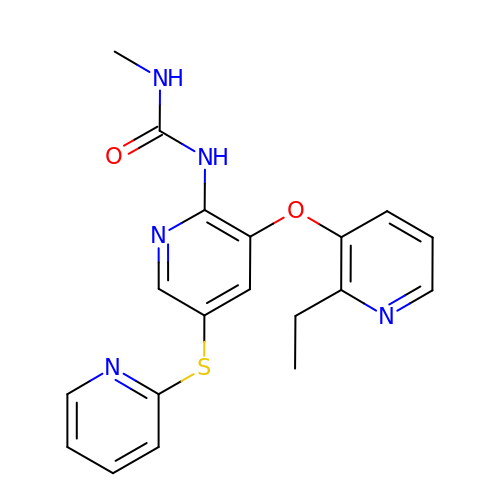1-{3-[(2-ethylpyridin-3-yl)oxy]-5-(pyridin-2-ylsulfanyl)pyridin-2-yl}-3-methylurea | C19 H19 N5 O2 S | PIGWQTQWPKNWHF-UHFFFAOYSA-N>M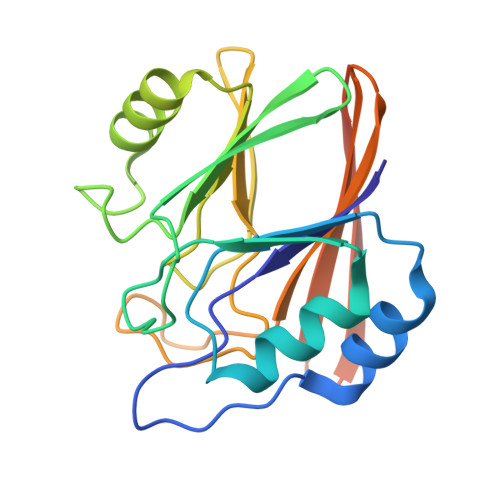LVLVIGDFHVPHRSAAIPQVFLDRLNTGRIQTVLCTGNLCGKETYDILRTLAREVHVVKGAFDEMQGLNETEVIKIGNFKIGLMHGHQVIPWGDREALAIYQRQLDVDILITGHTHKLETKEVGGKYFLNPGSATGAYSPLVDNPVPSFMLLEINDSELTIYEYTLVDGSVKCERVDFNKKQQQLEHHHHHH[2x]> APGEEDLCAAFNVICDNVGKDWRRLARQLKVSDTKIDSIEDRYPRNLTERVRESLRIWKNTEKENATVAHLVGALRS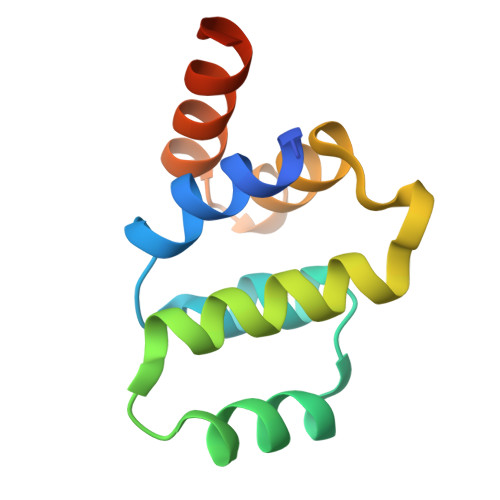CQMNLVADLVQEVQQARDLQNRSG>[4x]MDTKLYIDGQWVNSSSGKTVDKYSPVTGQVIGRMEAATRDDVDRAIDAAEDAFWAWNDLGSVER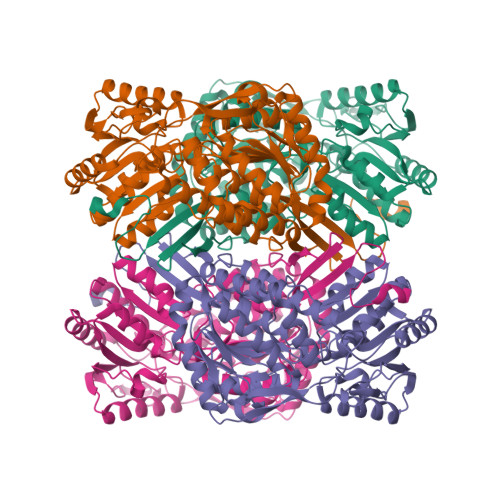SKIIYRAKELIEKNRAELENIIMEENGKPVKEAKEEVDGVIDQIQYYAEWARKLNGEVVEGTSSHRKIFQYKVPYGIVVALTPWNFPAGMVARKLAPALLTGNTVVLKPSSDTPGSAEWIVRKFVEAGVPKGVLNFITGRGSEIGDYIVEHKKVNLITMTGSTATGQRIMQKASANMAKLILELGGKAPFMVWKDADMDNALKTLLWAKYWNAGQSCIAAERLYVHEDIYDTFMSRFVELSRKLALGDPKNADMGPLINKGALQATSEIVEEAKESGAKILFGGSQPSLSGPYRNGYFFLPTIIGNADQKSKIFQEEIFAPVIGARKISSVEEMYDLANDNKYGLASYLFTKDPNIIFEASERIRFGELYVNMPGPEASQGYHTGFRMTGQAGEGSKYGISEYLKLKNIYVDYSGKPLHINTVRDDLFQSGRPVLGSSHHHHHH His domain protein tyrosine phosphatase (HD-PTP/PTPN23) is a tumor suppressor that regulates mitogenic receptor downregulation, endocytic recycling, and cell migration (Chen et al., 2012, Doyotte et al., 2008, Kharitidi et al., 2015, Lee et al., 2007, Ma et al., 2015, Manteghi et al., 2016). A central feature of HD-PTP function is the ability of its Bro1 domain to recruit CHMP4, the major subunit of the ESCRT-III membrane remodeling protein complex (Doyotte et al., 2008, Ichioka et al., 2007, Parkinson et al., 2015). Crystallographic structures of the HD-PTPBro1 domain in complex with the relevant binding regions of SARA, endofin, and all three human CHMP4 isoforms reveal that SARA and endofin binding is similar to that of CHMP4 at the conserved site, but critically extends into a neighboring specific pocket unique to HD-PTP. Altogether, this study identifies the Bro1 domain of HD-PTP as a highly selective interaction hub that coordinates recruitment of endosomal signaling adaptors versus MVB sorting and receptor degradation.

We then demonstrated by biosensor binding experiments that the first 22 residues of endofin, bound to HD-PTPBro1 and HD-PTPBro1-CC with similar high affinity (dissociation constant KD 3.1 ± 0.1 μM and 2.7 ± 0.1 μM, respectively), suggesting that the endofin binding site is in the Bro1 domain of HD-PTP. As predicted, the 22-mer SARA/endofin peptides form amphipathic α helices in their complexes with HD-PTPBro1. They occupy a larger binding site than the CHMP4 peptides, partially overlapping with the common site across H5, H6, and H7, but extending further into the S site between H3 and H5. The SARA/endofin-HD-PTPBro1 binding interface is largely hydrophobic and involves residues F5, A9/V9, L12, L16, and F19 present in both peptides. Leu16 accommodates itself into the second hydrophobic pocket and interacts with L202/I206 in the endofin-HD-PTPBro1 complex and I206 in the SARA-HD-PTPBro1 complex, consistent with the importance of these residues for SARA/endofin binding to HD-PTP. The crystal structures explain the impaired binding to HD-PTPBro1 shown by L15P and L15E mutants of endofin. L15 forms hydrophobic interactions with L338 at the proline-rich C-terminal region of HD-PTPBro1. Substitution by Glu would disrupt these interactions and also clash with L338, whereas substitution by Pro may cause a disruption of the helical structure and potentially result in the loss of several interactions at either side. Another key interaction in the S site is the hydrogen bond between the hydroxyl group of Y4 in SARA/endofin and D348 in HD-PTPBro1. Indeed, a shorter endofin peptide lacking 1-MDSYF-5 showed poor binding (>1.5 mM) to HD-PTPBro1 or HD-PTPBro1-CC, confirming the importance of the Y4 and F5 interactions.

>MEAVPRMPMIWLDLKEAGDFHFQPAVKKFVLKNYGENPEAYNEELKKLELLRQNAVRVPRDFEGCSVLRKYLGQLHYLQSRVPMGSGQEAAVPVTWTEIFSGKSVAHEDIKYEQACILYNLGALHSMLGAMDKRVSEEGMKVSCTHFQCAAGAFAYLREHFPQAYSVDMSRQILTLNVNLMLGQAQECLLEKSMLDNRKSFLVARISAQVVDYYKEACRALENPDTASLLGRIQKDWKKLVQMKIYYFAAVAHLHMGKQAEEQQKFGERVAYFQSALDKLNEAIKLAKGQPDTVQDALRFTMDVIGGKYNSAKKDNDFIYHEAVPALDTLQPVKGAPLVKPLPVNPTDPAVTGPDIFAKLV[2x];>MDSYFKAAVSDLDKLLDDFEQN[2x]> MKESYYSIGEVSKLANVSIKALRYYDKIDLFKPAYVDPDTSYRYYTDSQLIHLDLIKSLKYIGTPLEEMKKAQDLEMEELFAFYTEQERQIREKLDFLSALEQTISLVKKRMKR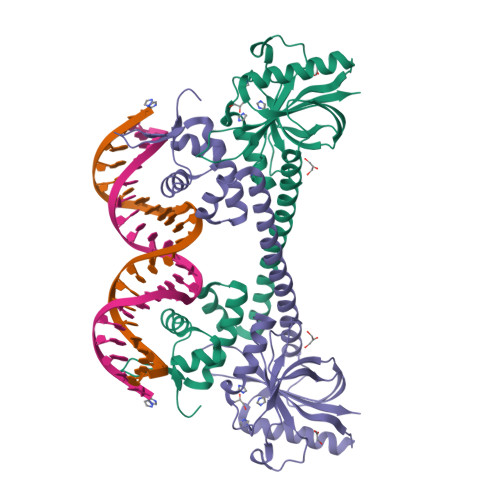QMEYPALGEVFVLDEEEIRIIQTEAEGIGPENVLNASYSKLKKFIESADGFTNNSYGATFSFQPYTSIDEMTYRHIFTPVLTNKQISSITPDMEITTIPKGRYACIAYNFSPEHYFLNLQKLIKYIADRQLTVVSDVYALIIPIHYSPKKQEEYRVEMKIRILDHHHHHH> MRDTRFPCLCGIAASTLLFATTPAIAGEAPADRLKALVDAAVQPVMKANDIPGLAVAISLKGEPHYFSYGLASKEDGRRVTPETLFEIGSVSKTFTATLAGYALAQDKMRLDDRASQHWPALQGSRFDGISLLDLATYTAGGLPLQFPDSVQKDQAQIRDYYRQWQPTYAPGSQRLYSNPSIGLFGYLAARSLGQPFERLMEQQVFPALGLEQTHLDVPEAALAQYAQGYGKDDRPLRVGPGPLDAEGYGVKTSAADLLRFVDANLHPERLDRPWAQALDATHRGYYKVGDMTQGLGWEAYDWPISLKRLQAGNSTPMALQPHRIARLPAPQALEGQRLLNKTGSTNGFGAYVAFVPGRDLGLVILANRNYPNAERVKIAYAILSGLEQQGKVPLKR

Pseudomonas aeruginosa is a major gram-negative pathogen responsible for a variety of infections and possessing an array of both intrinsic and acquired resistance mechanisms, including β-lactamases, like the chromosomal Pseudomonas-derived cephalosporinase (PDC). β-Lactams are the most widely prescribed class of antibiotics in the United States, and antipseudomonal cephalosporins (including cefepime) are important therapies (alone or combined with β-lactamase inhibitors) for P. aeruginosa infections. Taniborbactam (formerly VNRX-5133) is a novel, investigational, bicyclic boronate β-lactamase inhibitor shown to inhibit members of all four Ambler classes of β-lactamase enzymes. PDC-88 was chosen as a representative member of the group for detailed characterization and is noted for a T289-P290 deletion (by structural alignment-based numbering of class C β-lactamases, “SANC”) in the R2-loop (ΔT289-P290). Herein, we focus our efforts on PDC-88 to better understand both the basis of this expanded-spectrum activity and its inhibition by taniborbactam.

The active sites of the PDC-3 and PDC-88 structures in complex with taniborbactam revealed strong electron density for the bicyclic boronic acid inhibitor. Taniborbactam was covalently bonded to the hydroxyl group of the PDC catalytic serine (S64 by SANC) and made extensive interactions in both the PDC-3 and PDC-88 active sites. The boronic hydroxyl moiety of taniborbactam in both complexes made hydrogen bonds with the backbone nitrogen atoms in the oxyanion hole involving residues S64 and S318, as well as with the backbone oxygen of S318. The carboxyl moiety of taniborbactam interacted with T316 and S318; the amide moiety of taniborbactam made hydrogen bonds across the width of the active site (with the backbone oxygen of S318 and with the side chains of N152). The hydrophobic bicyclic rings of taniborbactam made hydrophobic interactions in the active sites with L119, Y150, and L293. For PDC-3, residues Y150 and Q120 adopted two conformations in the apo structures and only one conformation when taniborbactam was bound. We superimposed and compared the taniborbactam-bound structures of the Class A CTX-M-15 (10), Class C E. coli AmpC, and Class D OXA-10 (34) with PDC-3. The major difference in taniborbactam conformation between PDC-3 and the other three structures is found in the 2-aminoethylamino-cyclohexyl moiety. In PDC-3, this moiety extends away from the bicyclic scaffold moiety, whereas in CTX-M-15, AmpC, and OXA-10, this moiety points in a different direction, allowing it to make van der Waals interaction with the hydrophobic atoms of the bicyclic scaffold of taniborbactam.7-ethyl-6-[(3-methoxyphenyl)sulfanyl]-5-methyl-7H-pyrrolo[2,3-d]pyrimidine-2,4-diamine 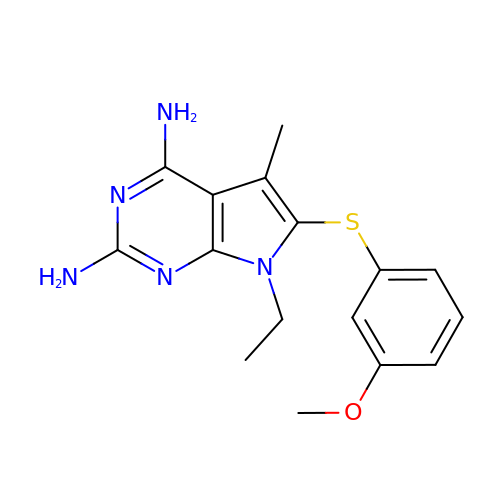| C16 H19 N5 O S | ULDSMDKWSKBCEI-UHFFFAOYSA-N> MAVTDLRDVEEDVKGKLDEWLNALVHLDKQQVERIYEELQGEMKHVLDFEIINYYKLLYTRYLIMKRDISALEEELDKLKKVYKKYSPFQKLLYMYGRGLLCCLQYRWKDGLDYLLKTEVMAKEQGYHETGLYYNIALAYTHLDIHHLAIHFVNMALEGFRSEYKFRNIINCQILIAVSYTEKGQYEEALKMYESILREATSFADKDVLLAITLSNMGSIYYKKGKYQQAKKYYLDSLQLQKQIDLNYLDTIYEMALVCIKLEELEEART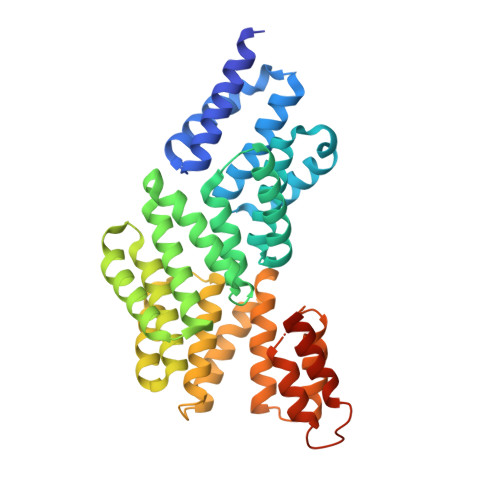LIDKGIDAAKQEERFNAKLYLLLMLRYKYFEEAKDYKAFLENEAIPLYKSAGNKIELKKVYVELAEHFSSLSRFEESNRYYRLVIDLMNDNKEERSHHHHHH> GSDITRFLVK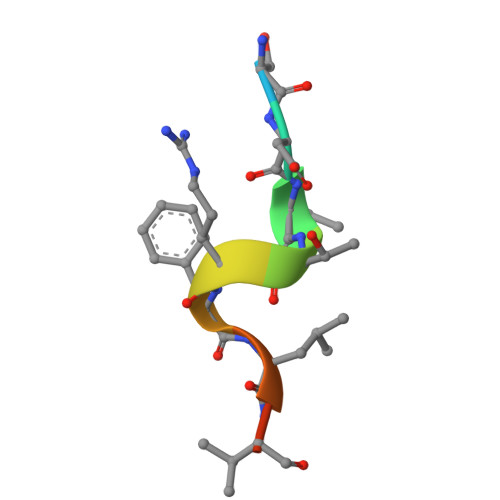K> AERSELTIHPKEFTTFVRNFNPFLGATNLHTTTDFIYEPLVVFNEMHGNTPVFRLAENFQMSDDLMSVTFDIRKGVKWSDGEAFTADDVVYSFNLVKEKPELDQSGINSWVTGVEKVNDYQVKFRLSEANSNVPYEIAKVPVVPKHVWSKVKDPSTFTNENPVGSGPFTVIDTFTPQLYIQCENPNYWDAANLDVDCLRVPQIANNDQFLGKVVNGEMDWTSSFVPDIDRTYAAASPKHHYWYPPAGTQAFVVNFKNPDAAKNEALTNVDFRRAFSMALDRQTIIDIAFYGGGTVNDFASGLGYAFEAWSDEKTHDKFKAYNSYNAEGAKKLLAKAGFKDVNKDGFVDTPSGKSFELLIQSPNGWTDFNNTVQLAVEQLAEVGIKARARTPDFSVYNQAMLEGTYDVAYTNYFHGADPYTYWNSAYNSALQSGDGMPRFAMHFYKNEKLDGLLNSFYKTADKQEQLEIAHGIQQIIAQDQVTIPVLSGAYMYQYNTTRFTGWWNEENPKGRPNIWA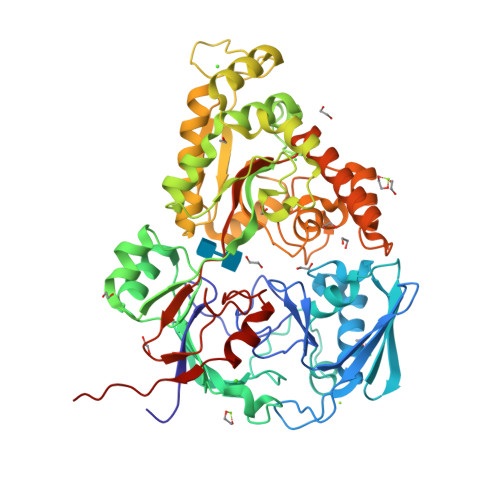GIPERLLHVLDLKPVKLEHHHHHH> GGACACUGAUGAUCGCGUGGAUAUGGCACGCAUU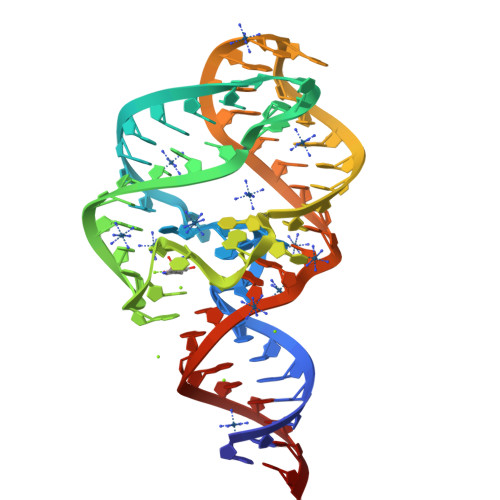GAAUUGUUGGACACCGUAAAUGUCCUAACACGUGUCC> DSSIKRTANINLYKLDQRFKQSRINIESFHSTVLLTGQVPDPY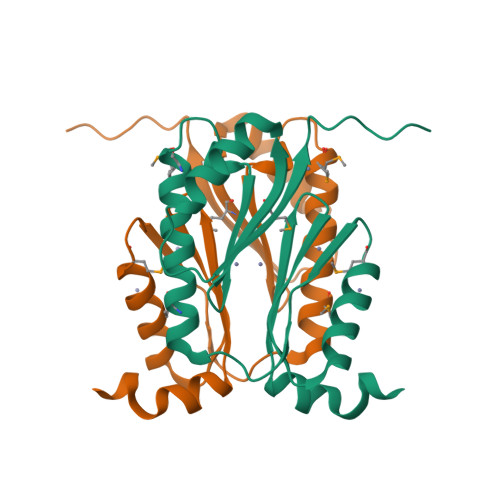LKQLAEDNVKAMSDVKAVHNYITVGNKVSYNTIMQDAGVTANTRALLMKAPVVSDSKVLVHTEDGVLYVMGRLNTAEINDLNNVLQNVGNVTKIVTLIDNIDLAPAPAASTASATTTPVINNVLAQPTVQTPVAIDPDQTDPASSAQ>[2x]MHHHHHHSSGRENLYFQGKMWKPGD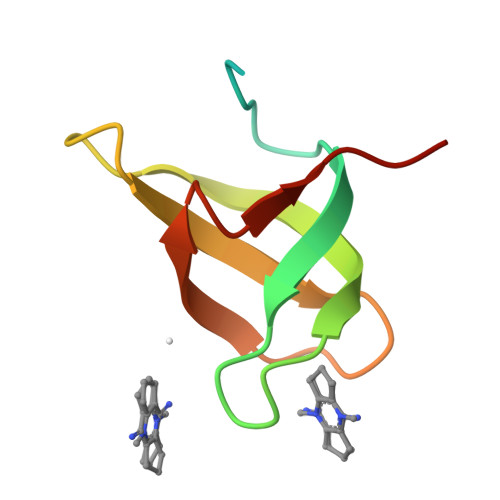ECFALYWEDNKFYRAEVEALHSSGMTAVVKFIDYGNYEEVLLSNIKPIQTE>[2x]MDTPNKDDSIIRFSVSLQQNLLDELDNRIIKNGYSSRSELVRDMIREKLVEDNWAEDNPNDESKIAVLVVIYDGGQRELNQRMIDIQHASGTHVLCTTHIHMDEHNCLETIILQGNSFE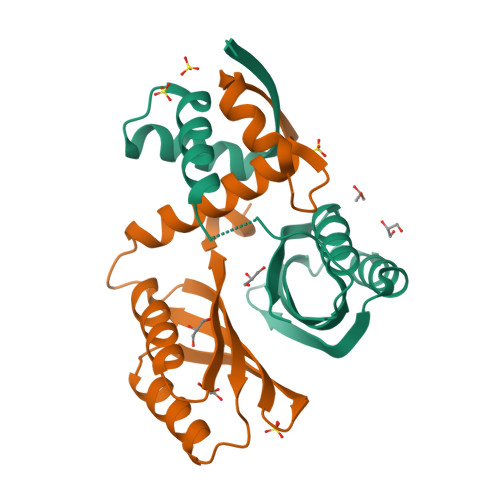IQRLQLEIGGLRGVKFAKLTKASSFEYNE> AGSAPLLLYANRRDLRLVDATNGKENATIVVGGLEDAAAVDFVFSHGLIYWSDVSEEAIKRTEFNKTESVQNVVVSGLLSPDGLACDWLGEKLYWTDSETNRIEVSNLDGSLRKVLFWQELDQPRAIALDPSSGFMYWTDWGEVPKIERAGMDG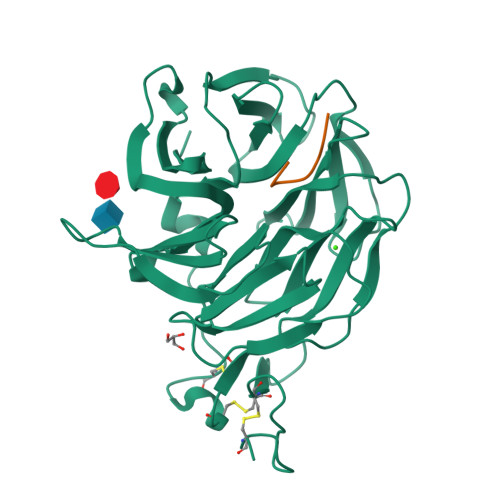SSRFIIINSEIYWPNGLTLDYEEQKLYWADAKLNFIHKSNLDGTNRQAVVKGSLPHPFALTLFEDILYWTDWSTHSILACNKYTGEGLREIHSDIFSPMDIHAFSQQRQPNATNPCGIDNGGCSHLCLMSPVKPFYQCACPTGVKLLENGKTCKDGNSHHHHHH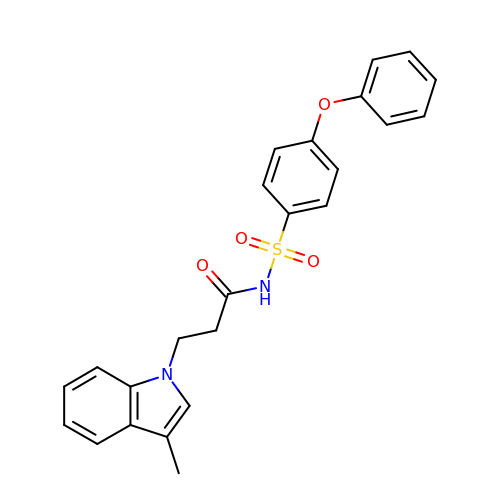3-(3-methylindol-1-yl)-~{N}-(4-phenoxyphenyl)sulfonyl-propanamide | C24 H22 N2 O4 S | ZPEFTTKCRHGFDO-UHFFFAOYSA-N>TTVNETTPIAPAKVLPDAQTVTSVRHWTDTLFSFRVTRPQTLRFRSGEF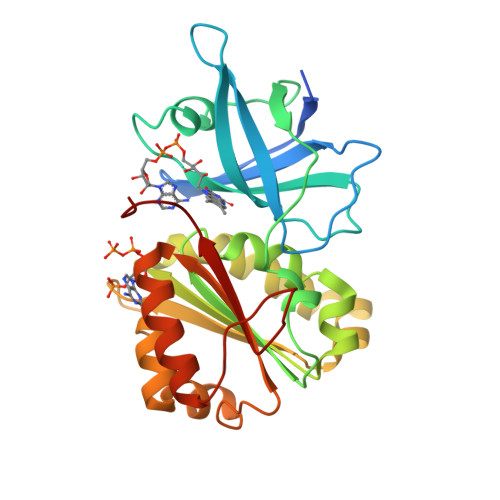VMIGLLDDNGKPIMRAYSIASPAWDEELEFYSIKVPDGPLTSRLQHIKVGEQIILRPKPVGTLVIDALLPGKRLWFLATGTGIAPFASLMREPEAYEKFDEVIMMHACRTVAELEYGRQLVEALQEDPLIGELVEGKLKYYPTTTREEFHHMGRITDNLASGKVFEDLGIAPMNPETDRAMVCGSLAFNVDVMKVLESYGLREGANSEPREFVVEKAFVGEGI[4x]>DSLGWSNVDVLDRICEAYGFSQKIQLANHFDIASSSLSNRYTRGAISYDFAAHCALETGANLQWLLTGEGEAFVNNRESSDAKRIEGFTLSEEILKSDKQLSVDAQFFTKPLTDGMAIRSEGKIYFVDKQASLSDGLWLVDIKGAISIRELTKLPGRKLHVAGGKVPFECGIDDIKTLGRVVGVY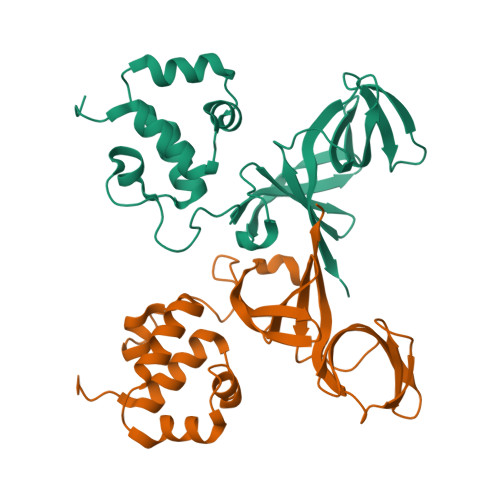SEVN[2x]benzyl (cyanomethyl)carbamate 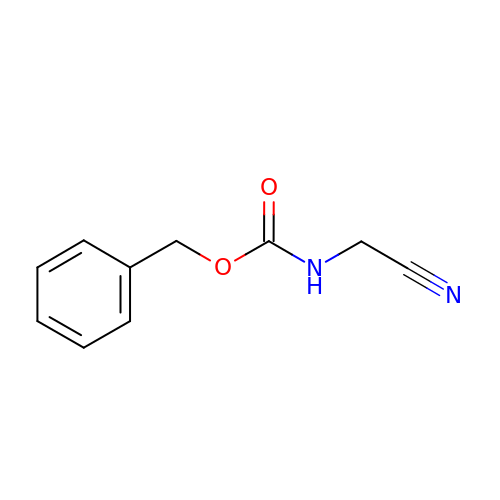| C10 H10 N2 O2 | DVUXKEFDAGQPQU-UHFFFAOYSA-N Integration of retroviral DNA by the viral integrase (IN) into cellular DNA is a necessary step for virus replication. RSV IN is homodimeric in solution. The 3′ OH cleavage of blunt-ended viral DNA by IN yields intasomes with recessed ends, here termed the cleaved synaptic complex (CSC). We determined the structure of RSV octameric intasome stabilized by a HIV-1 IN strand transfer inhibitor using single particle cryo-electron microscopy.

Thus, we determined the structure of the octameric CSC formed with IN 1–278 and GU3 18R viral DNA in the presence of INSTI MK-2048 by single-particle cryo-EM. The final map had an overall resolution of 3.2 Å and local resolution reaching ~2.8 Å for the core region of the complex containing the two IN catalytic sites bound with INSTIs and viral DNA, which was significantly improved from the previously reported RSV STC X-ray crystal structure that was determined at 3.8 Å resolution. Well-defined cryo-EM density was observed for both of the proximal IN dimers, all four CTDs of both distal (flanking) IN dimers, two viral DNAs, and the two MK-2048 molecules occupying the active sites of the inner catalytic IN molecules. IN residues downstream from Ile269 were not discernable in the EM map. The cryo-EM map of the CSC structure shows that the CCD of the distal IN dimers position farther away from the CIC region, rendering a more cruciform-like, overall open conformation of the CSC when viewed along the pseudo twofold axis. The NTDs associated with these CCDs were not modeled due to low-quality density in these regions. Weaker and less well-defined density compared to the rest of the complex suggested that the NTDs and CCDs of the distal IN dimers are highly flexible in the absence of target DNA. MK-2048, the INSTI included during complex formation, is bound at the interface between IN and the viral DNA 3′ terminus, sequestering the two magnesium ions in the active site. The chloro-fluorobenzyl moiety stacks on the penultimate cytosine base of the terminal CA dinucleotide motif, displacing the terminal deoxyadenosine (dA). The displaced dA in turn stacks on the core metal-coordinating ring system of MK-2048. Notably, Arg263 from the CTD of a distal IN subunit, which bridges between the CCD and CTD of the catalytic IN molecule as part of the CIC, interacts with the Gln151 side chain as well.

>[8x]PLREAKDLHTALHIGPRALSKACNISMQQAREVVQTCPHCNSAPALEAGVNPRGLGPLQIWQTDFTLEPRMAPRSWLAVTVDTASSAIVVTQHGRVTSVAVQHHWATAIAVLGRPKAIKTDNGSCFTSKSTREWLARWGIAHTTGIPGNSQGQAMVERANRLLKDKIRVLAEGDGFMKRIPTSKQGELLAKAMYALNHFERGENTKTPIQKHWRPTVLTEGPPVKIRIETGEWEKGWNVLVWGRGYAAVKNRDTDKVIWVPSRKVKPDITQKDEVTKK> EGYGKHITSMHVRNIFNQGNQVIRNIVKQQRYELLDFTGT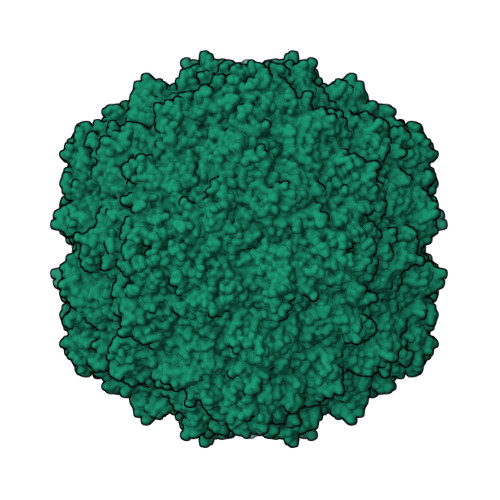EAGTTNLPKIIPYQCIWWRGLQNAANVNQTINNMIALNTISYGVRFLKAKLCIEVYAVTRKRLIQTGATSYYTDDFEQGQNLFIGWADRKAESIPITTPADLDETKLTVANTTLFDANNDNITKEEVPTREKWCHTWDLDVLNHNYLWEPNNLDSQWTLIPGAQAVQPTATPIGPTYQEIVIATKAIGANESALVTTIQDRRSYPRLMLSQPQIKDETDTMKFKYQIRISTELEMEHHIKPDIANPWLTRQTLPLPALSGDGTTRYVPCVPYETHVSQ> MGRLLALVVGAALVSSACGGCVEVDSETEAVYGMTFKILCISCKRRSETNAETFTEWTFRQKGTEEFVKILRYENEVLQLEEDERFEGRVVWNGSRGTKDLQDLSIFITNVTYNHSGDYECHVYRLLFFENYEHNTSVVKKIHIEVVDKANRDMASIVSEIMMYVLIVVLTIWLVAEMIYCYKKIAAATETAAQENASEYLAITSESKENCTGVQVAE;> MHRDAWLPRPAFSLTGLSLFFSLV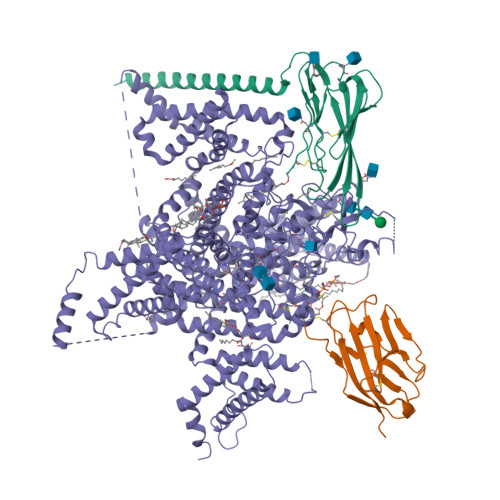PPGRSMEVTVPATLNVLNGSDARLPCTFNSCYTVNHKQFSLNWTYQECNNCSEEMFLQFRMKIINLKLERFQDRVEFSGNPSKYDVSVMLRNVQPEDEGIYNCYIMNPPDRHRGHGKIHLQVLMEEPPERDSTVAVIVGASVGGFLAVVILVLMVVKCVRRKKEQKLSTDDLKTEEEGKTDGEGNPDDGAK;> MAQALLVPPGPESFRLFTRESLAAIEKRAAEEKAKKPKKEQDNDDENKPKPNSDLEAGKNLPFIYGDIPPEMVSEPLEDLDPYYINKKTFIVMNKGKAIFRFSATSALYILTPLNPVRKIAIKILVHSLFSMLIMCTILTNCVFMTLSNPPDWTKNVEYTFTGIYTFESLIKILARGFCLEDFTFLRDPWNWLDFSVIVMAYVTEFVSLGNVSALRTFRVLRALKTISVIPGLKTIVGALIQSVKKLSDVMILTVFCLSVFALIGLQLFMGNLRNKCLQWPPSDSAFETNTTSYFNGTMDSNGTFVNVTMSTFNWKDYIGDDSHFYVLDGQKDPLLCGNGSDAGQCPEGYICVKAGRNPNYGYTSFDTFSWAFLSLFRLMTQDYWENLYQLTLRAAGKTYMIFFVLVIFLGSFYLVNLILAVVAMAYEEQNQATLEEAEQKEAEFQQMLEQLKKQQEEAQAVAAASAASRDFSGIGGLGELLESSSEASKLSSKSAKEWRNRRKKRRQREHLEGNNKGERDSFPKSESEDSVKRSSFLFSMDGNRLTSDKKFCSPHQSLLSIRGSLFSPRRNSKTSIFSFRGRAKDVGSENDFADDEHSTFEDSESRRDSLFVPHRHGERRNSNVSQASMSSRMVPGLPANGKMHSTVDCNGVVSLVGGPSALTSPTGQLPPEGTTTETEVRKRRLSSYQISMEMLEDSSGRQRAVSIASILTNTMEELEESRQKCPPCWYRFANVFLIWDCCDAWLKVKHLVNLIVMDPFVDLAITICIVLNTLFMAMEHYPMTEQFSSVLTVGNLVFTGIFTAEMVLKIIAMDPYYYFQEGWNIFDGIIVSLSLMELGLSNVEGLSVLRSFRLLRVFKLAKSWPTLNMLIKIIGNSVGALGNLTLVLAIIVFIFAVVGMQLFGKSYKECVCKINDDCTLPRWHMNDFFHSFLIVFRVLCGEWIETMWDCMEVAGQTMCLIVFMLVMVIGNLVVLNLFLALLLSSFSSDNLAATDDDNEMNNLQIAVGRMQKGIDYVKNKMRECFQKAFFRKPKVIEIHEGNKIDSCMSNNTGIEISKELNYLRDGNGTTSGVGTGSSVEKYVIDENDYMSFINNPSLTVTVPIAVGESDFENLNTEEFSSESELEESKEKLNATSSSEGSTVDVVLPREGEQAETEPEEDLKPEACFTEGCIKKFPFCQVSTEEGKGKIWWNLRKTCYSIVEHNWFETFIVFMILLSSGALAFEDIYIEQRKTIKTMLEYADKVFTYIFILEMLLKWVAYGFQTYFTNAWCWLDFLIVDVSLVSLVANALGYSELGAIKSLRTLRALRPLRALSRFEGMRVVVNALVGAIPSIMNVLLVCLIFWLIFSIMGVNLFAGKFYHCVNMTTGNMFDISDVNNLSDCQALGKQARWKNVKVNFDNVGAGYLALLQVATFKGWMDIMYAAVDSRDVKLQPVYEENLYMYLYFVIFIIFGSFFTLNLFIGVIIDNFNQQKKKFGGQDIFMTEEQKKYYNAMKKLGSKKPQKPIPRPANKFQGMVFDFVTRQVFDISIMILICLNMVTMMVETDDQGKYMTLVLSRINLVFIVLFTGEFVLKLVSLRHYYFTIGWNIFDFVVVILSIVGMFLAEMIEKYFVSPTLFRVIRLARIGRILRLIKGAKGIRTLLFALMMSLPALFNIGLLLFLVMFIYAIFGMSNFAYVKKEAGIDDMFNFETFGNSMICLFQITTSAGWDGLLAPILNSAPPDCDPDTIHPGSSVKGDCGNPSVGIFFFVSYIIISFLVVVNMYIAVILENFSVATEESAEPLSEDDFEMFYEVWEKFDPDATQFIEFSKLSDFAAALDPPLLIAKPNKVQLIAMDLPMVSGDRIHCLDILFAFTKRVLGESGEMDALRIQMEDRFMASNPSKVSYEPITTTLKRKQEEVSAAIIQRNFRCYLLKQRLKNISSNYNKEAIKGRIDLPIKQDMIIDKLNG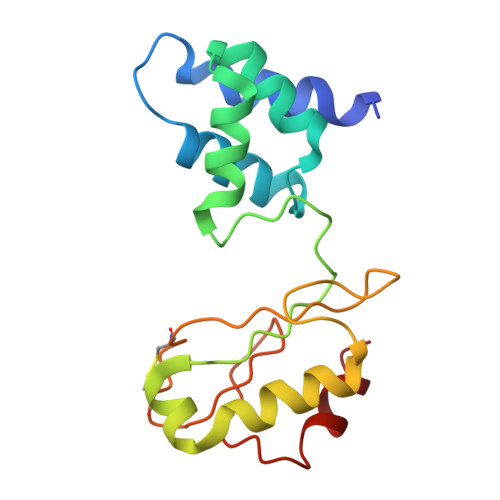> MALSTVDVVEKVKEIVAPWKGKQGGLIPILQEVQRELGYLPEEALLTISRELKMPKAEVYGVATFYAQFHLKPRGRHVIRVCRGTACHVRGSLQILEKVKQMLGIEENETTDDLRFTLEPVACLGACGLAPVMMVDEDTHGRMTPDKIQAILDKYQ>SVDDEPIRLPNPMIGFGVPNEPGLITHRSLPELARGPPFFYYENVALTPKGVWETISRHLFEIPPEFVDSKYFCVAARKRGYIHNLPINNRFQIQPPPKYTIHDAFPLSKRWWPEWDKRTKLNCILTCTGSAQLTNRIRVALEPYNEEPEPPKHVQRYVIDQCKKWNLVWVGKNKAAPLEPDEMESILGFPKNHTRGGGMSRTERFKSLGNSFQVDTVAYHLSVLKPIFPHGINVLSLFTGIGGGEVALHRLQIKMKLVVSVE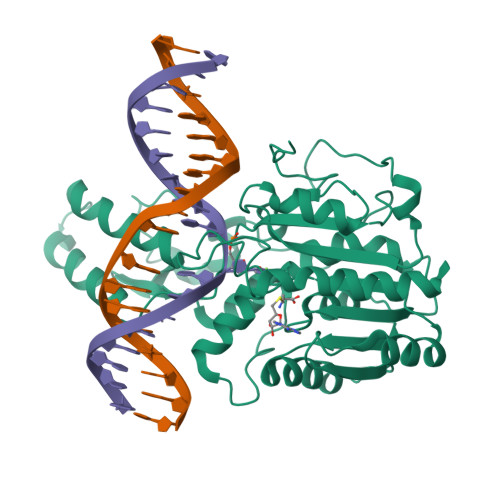ISKVNRNILKDFWEQTNQTGELIEFSDIQHLTNDTIEGLMEKYGGFDLVIGGSPCNNLAGGNRVSRVGLEGDQSSLFFEYCRILEVVRARMRGS[2x]> MEYGHHARPDSKRPLDEGSPAAAGLTSKKANEALTRNRELTTVLVKNLPKSYNQNKVYKYFKHCGPIIHVDVADSLKKNFRFARIEFARYDGALAAITKTHKVVGQNEIIVSHLTECTLWMTNFPPSYTQRNIRDLLQDINVVALSIRLPSLRFNTSRRFAYIDVTSKEDARYCVEKLNGLKIEGYTLVTKVSNPLEKSKRTDSATLEGREIMIRNLSTELLDENLLRESFEGFGSIEKINIPAGQKEHSFNNCCAFMVFENKDSAERALQMNRSLLGNREISVSLADKKPFLERNEVKRLLASRNSKELETLICLFPLSDKVSPSLICQFLQEEIHINEKDIRKILLVSDFNGAIIIFRDSKFAAKMLMILNGSQFQGKVIRSGTINDMKRYYNNQQNHSMKHVKPSCINMMEKGPNLQVKKKIPDKQEQMSNDDFRKMFLGELEHHHHHH;> MGSMLFFSFFKTLVDQEVVVELKNDIEIKGTLQSVDQFLNLKLDNISCTDEKKYPHLGSVRNIFIRGSTVRYVYLNKNMVDTNLLQDATRREVMTERK;> MGSMETPLDLLKLNLDERVYIKLRGARTLVGTLQAFDSHCNIVLSDAVETIYQLNNEELSESERRCEMVFIRGDTVTLISTPSEDDDGAVEI;> MGSMLPLYLLTNAKGQQMQIELKNGEIIQGILTNVDNWMNLTLSNVTEYSEESAINSEDNAESSKAVKLNEIYIRGTFIKFIKLQDNIIDKVKQQI;> MGSMSLPEILPLEVIDKTINQKVLIVLQSNREFEGTLVGFDDFVNVILEDAVEWLIDPEDESRNEKVMQHHGRMLLSGNNIAILVPGGKKTPTEAL;> GSMSGKASTEGSVTTEFLSDIIGKTVNVKLASGLLYSGRLESIDGFMNVALSSATEHYESNNNKLLNKFNSDVFLRGTQVMYISEQKI;> MGSMHQQHSKSENKPQQQRKKFEGPKREAILDLAKYKDSKIRVKLMGGKLVIGVLKGYDQLMNLVLDDTVEYMSNPDDENNTELISKNARKL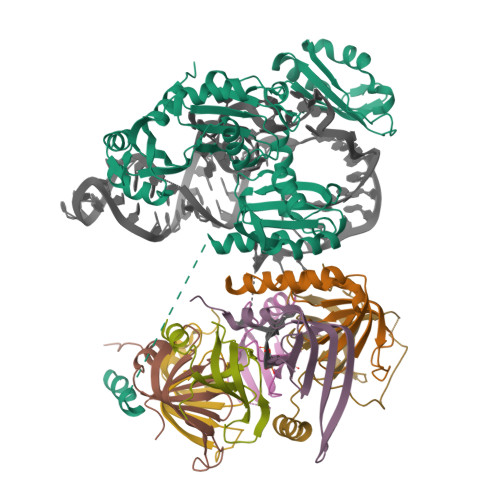GLTVIRGTILVSLSSAEGSDVLYMQK;> GSMSATLKDYLNKRVVIIKVDGECLIASLNGFDKNTNLFITNVFNRISKEFICKAQLLRGSEIALVGLIDAENDDSLAPIDEKKVPMLKDTKNKIENEHVIWEKVYESKTK>GSHFEEGERVLAKHSDCFYEAKVLKVEFKDNEWKYFVHYIGWNKSWDEWIRLDCLLKHSDENIEKQKEQGLKQQG[2x];>[2x]ATGGVKKPHRY

MRG1 and MRG2 belong to the MRG protein family, with highly conserved members in fungi, plants, and animals. Members in this group have the same domain organization, with a chromodomain (chromatin organization modifier domain) near the N-terminus, and a MRG domain near the C-terminus. Firstly, via their chromodomain, MRG1/2 proteins act as readers that recognize methylated H3K4 and H3K36. In addition, MRG1/2 proteins bind to chromatin that contains tri-methylated H3K4 and H3K36 via their chromodomains, the bound MRG1/2 in turn stabilize the binding of CO and ultimately controls the activation of FT transcription.

H3K4me3 (residues 1–9) and H3K36me3 (residues 31–41) exhibited detectable binding to MRG2 chromodomain (residues 41–123) (Kd values: 0.8 mM for H3K4me3; 0.69 mM for H3K36me3). To obtain the information regarding the specific MRG2 residues that are important for recognition of the histone marks H3K4me3 and H3K36me3, we determined the co-crystal structure of MRG2 and the methylated H3 peptides. The proteolyzed samples were analyzed using mass spectrometry (MS) analysis to determine the protein sequence, resulting in the identification of a region containing the chromodomain with residues 53–123 of MRG2 as suitable for crystallization. MRG2 complexes with the H3K4me3 and H3K36me3 peptides were obtained, but the complexes with the H3K27me3 and H3K9me3 peptides could not form crystals under the same conditions, consistent with the ITC results. The crystals of MRG2 with H3K4me3 or H3K36me3 were diffracted to 1.68 and 1.65 Å, respectively. In both structures, the MRG2 chromodomain contains mainly four beta-strands. However, the predicted alpha-helix located at the C-terminus is missing in the electron density map. For the complexes of the MRG2 chromodomain with the H3K4me3/H3K36me3 peptides, the recognition modes are almost the same; therefore, only the complex of the MRG2 chromodomain with H3K36me3 peptide is shown in Figure 7A. The tri-methylated lysine projects into the aromatic cage formed by the His62, Tyr67, Tyr87, Trp90, and Trp94 residues of the MRG2 chromodomain. The co-crystal structures clearly indicate that the chromodomain of MRG2 can directly bind to tri-methylated H3K4 and H3K36, and provide strong evidence that the aromatic cage of the MRG2 chromodomain and the associated residues are essential for the binding, the same as other chromodomain proteins. Consistent with the structure, the Tyr87Ala (Y87A) mutation in MRG2 disrupted its association with H3K4me3 and H3K36me3 peptides, supporting the idea that the hydrophobic pocket formed by the aromatic residues is essential for the binding, as with other chromodomain proteins.>LLIGVATSSLALHAPSQIVAAIKSRADQLGASVVVSMVERSGVEACKAAVHNLLAQRVSGLIINYPLDDQDAIAVEAACTNVPALFLDVSDQTPINSIIFSHEDGTR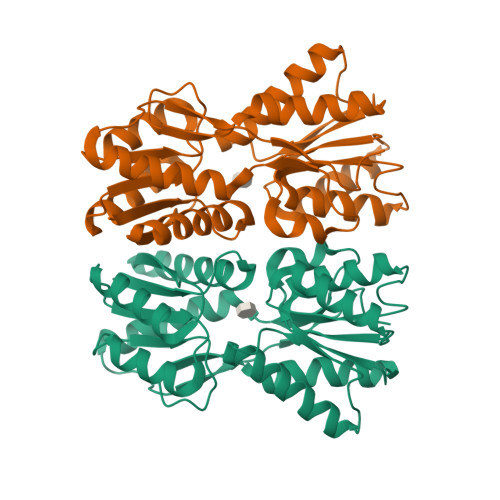LGVEHLVALGHQQIALLAGPLSSVSARLRLAGWHKYLTRNQIQPIAEREGDWSAMSGFQQTMQMLNEGIVPTAMLVANDQMALGAMRAITESGLRVGADISVVGYDDTEDSSCYIPPLTTIKQDFRLLGQTSVDRLLQLSQGQAVKGNQLLPVSLVKRKTTL[2x]>[2x]TPGTLLQESLLPREANYLAAIATGDGWGLAFLDVSTGEFKGTVLKSKSALYDELFRHRPAEVLLAPELLENGAFLDEFRKRFPVMLSEAPFEPEGEGPLALRRARGALLAYAQRTQGGALSLQPFRFYDPGAFMRLPEATLRALEVFEPLRGQDTLFSVLDETRTAPGRRLLQSWLRHPLLDRGPLEARLDRVEGFVREGALREGVRRLLYRLADLERLATRLELGRASPKDLGALRRSLQILPELRALLGEEVGLPDLSPLKEELEAALVEDPPLKVSEGGLIREGYDPDLDALRAAHREGVAYFLELEERERERTGIPTLKVGYNAVFGYYLEVTRPYYERVPKEYRPVQTLKDRQRYTLPEMKEKEREVYRLEALIRRREEEVFLEVRERAKRQAE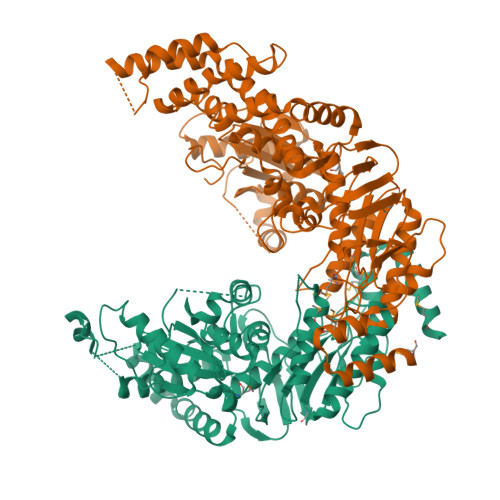ALREAARILAELDVYAALAEVAVRYGYVRPRFGDRLQIRAGRHPVVERRTEFVPNDLEMAHELVLITGPNMAGKSTFLRQTALIALLAQVGSFVPAEEAHLPLFDGIYTRIGASDDLAGGKSTFMVEMEEVALILKEATENSLVLLDEVGRGTSSLDGVAIATAVAEALHERRAYTLFATHYFELTALGLPRLKNLHVAAREEAGGLVFYHQVLPGPASKSYGVEVAAMAGLPKEVVARARALLQAMAAR> MKKITLLLAGSALLLSGCAGVKSSFDCDATTSDTCMTMTKANQLARDKAAKQAGKPAAGGLPSLVNLPATSAVEVPSASRSAVTPPSGTRTVSTTPPVSAGTSAGVNTNTTTSTLTPRPVAGTPVTTTPSSVAYRP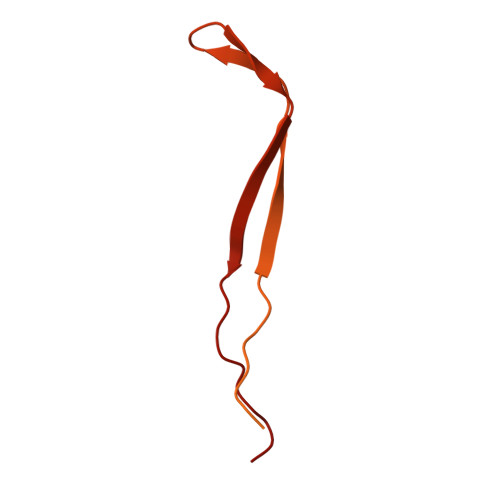VVSVVTPTPSCQNVRCDNPGTVHPQRSRDQIATVWIAPWVDSDNAFHQPGRVSFVVSPADWVLPARVN2-(1H-imidazol-1-yl)-N-(trans-4-methylcyclohexyl)acetamide | C12 H19 N3 O | 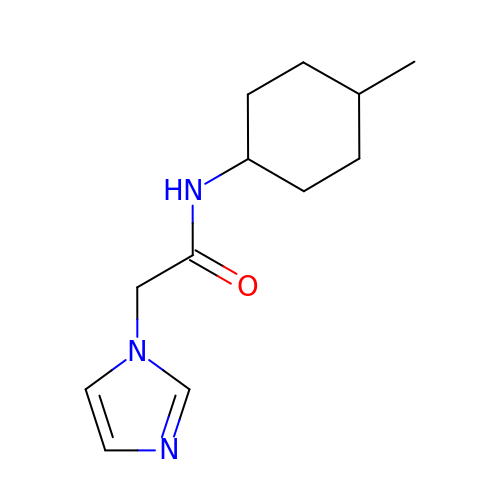PKHDTDLLHJFDKS-XYPYZODXSA-N N-[1-(2-chlorophenyl)-1H-indol-6-yl]-2-{[5-(2-chlorophenyl)-1H-tetrazol-1-yl]acetyl}hydrazinecarboxamide 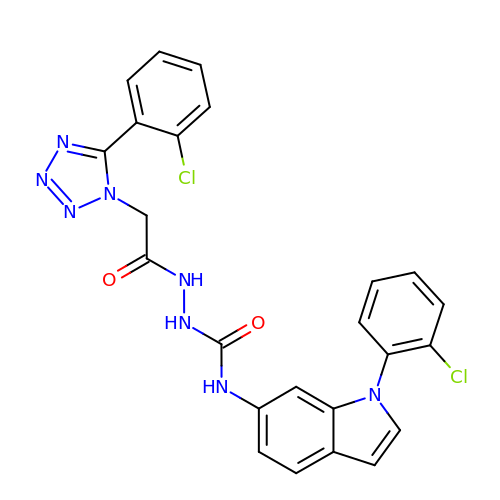| C24 H18 Cl2 N8 O2 | WJGUKFYAVSWTRD-UHFFFAOYSA-N> MADADPDVLKVALLPDENASELIKRNQPLKDYLEEHLDKKVQLIVTTDYSSMIEAMRFGRIDLAYFGPLSYVMAKSKSDIEPFAAMVIDGKPTYRSVIIANVASGVNEYADLKGKRMAYGDRASTSSHLIPKTVLLETADLTGGQDYEQHFVGTHDAVAVNVANGNADAGGLSEVIFNHAAERGLIDPSKVKVLGYSGEYPQYPWAMRSNLSPELKTKVRDVFVGIDDPEVLRNFKAE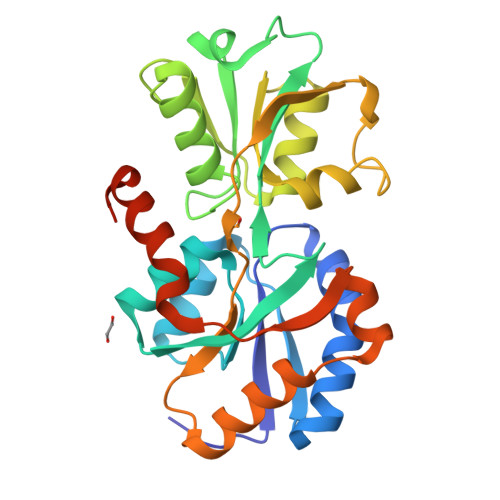AFAPITDADYDVIRNMGSLLGLDFATMLEHHHHHH>MIAPLLKTLPFLAAAYAAELDLPNFSALNRRQDNSTSSSAGCSLDQTVAPGNLTLCGNATLFTTFRPKARFIAPEGWMNAPMGLYQRADGSIHAGYQSHPKHIQWGNISQGAAYSS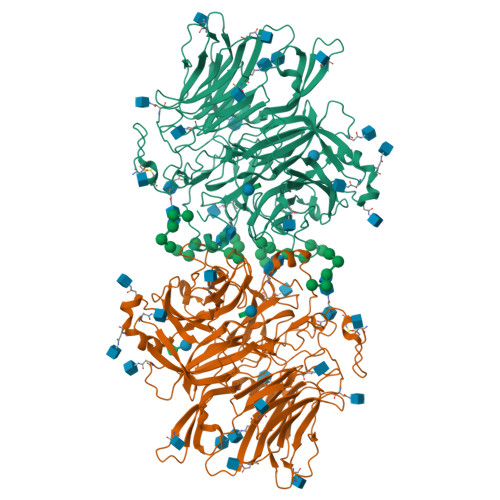DFTSWTDFNGSEGYKTIWPSQIYDIRGVFDGSIIKEGIDGYPTILYTSTSFGPLGATLNEAEGTETQSLAYTTDDGASWIKLGYGAGQNPVIYEWPETNLTGFRDPYVFQSPRLEALLANTTSITNATGDHFATISGGVHGDGARLFLYRQHTTGEFIKWTYLGPLVTTGYKESYGEWSGNYGINFETAGVTRLNPAGAAWDNGSDTTAVDFVTFGTEQGRADHQNHWPLWAAVDYEVRDNGSIEAVIAYSGVQDWGRSYAYASFPVEGYRQVSVGWIYEDDDNVILAKQFGYQGAFTLFRDLFVKVVENVSPSTPGLFEQASWSTKNSTDGMSVTVTTLGQRVVPETLAAYKGNSTVSTLAPVMLNESAAAYTPFSSQPTDRFYALTGSFEFGLNTTAKAGFRVLASEEEYTDIWFDPASENLTVVRTASSLIKSFGNDTELAKVKLYEIVGAESKTLNLTVFVDGSVIEIYANDEVALSTRAYPWLANSTGAGLLADGTTAGDVVGVSGLELWDGLVDAWPARPANTSQGLVWDGPTAAMYGLFAGY[2x]> MARVQFKQRESTDAIFVHCSATKPSQNVGVREIRQ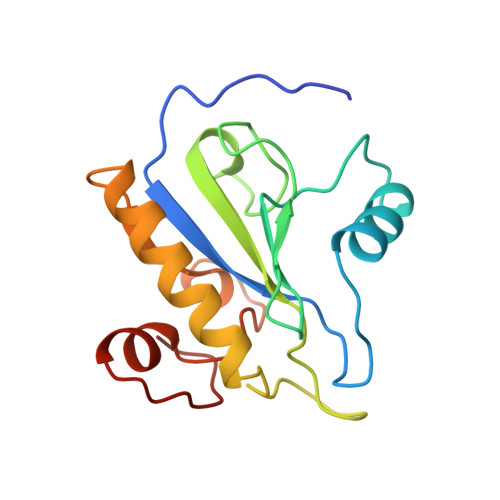WHKEQGWLDVGYHFIIKRDGTVEAGRDEMAVGSHAKGYNHNSIGVCLVGGIDDKGKFDANFTPAQMQSLRSLLVTLLAKYEGAVLRAHHEVAPKACPSFDLKRWWEKNELVTSDRG>GPGSRYPVRRLPFSTVSKQDLAAFERIVPGGVVTDPEALQAPNVDWLRTLRGCSKVLLRPRTSEEVSHILRHCHERNLAVNPQGGNTGMVGGSVPVFDEIILSTARMNRVLSFHSVSGILVCQAGCVLEELSRYVEERDFIMPLDLGAKGSCHIGGNVATNAGGLRFLRYGSLHGTVLGLEVVLADGTVLDCLTSLRKDNTGYDLKQLFIGSEGTLGIITTVSILCPPKPRAVNVAFLGCPGFAEVLQTFSTCKGMLGEILSAFEFMDAVCMQLVGRHLHLASPVQESPFYVLIETSGSNAGHDAEKLGHFLEHALGSGLVTDGTMATDQRKVKMLWALRERITEALSRDGYVYKYDLSLPVERLYDIVTDLRARLGPHAKHVVGYGHLGDGNLHLNVTAEAFSPSLLAALEPHVYEWTAGQQGSVSAEHGVGFRKRDVLGYSKPPGALQLMQQLKALLDPKGILNPYKTLPSQAHHHHHH[2x]

Human D-2-HGDH is a member of the 2-hydroxy acid dehydrogenase subfamily of the VAO/PCMH flavoprotein family. Regardless of their promiscuous metabolic origins, D-2-HG and L-2-HG can be converted back to 2-OG by two mitochondrial enzymes in humans, namely D-2-HG and L-2-HG dehydrogenases (D-2-HGDH and L-2-HGDH). Like other members of the VAO/PCMH flavoprotein family, D-2-HGDH is comprised of two major domains named the FAD-binding domain and the substrate-binding domain supplemented with a small C-terminal domain. The active site resides at the interface of the FAD-binding domain and the substrate-binding domain, and consists of the FAD-binding site and the substrate-binding site.

Crystallization of D-2-HGDH in the absence of any ligands yielded crystals of D-2-HGDH in apo form. Structure of the apo D-2-HGDH was solved at 2.20 Å resolution, and structures of D-2-HGDH in complexes with D-2-HG, D-MAL, D-LAC, L-2-HG, and 2-OG were solved at 2.65 Å, 2.80 Å, 2.62 Å, 3.00 Å, and 2.80 Å resolution, respectively. The asymmetric unit contains two D-2-HGDH molecules with essentially identical conformation. In all the structures, there is a FAD non-covalently bound to the active site, which is apparently co-purified with the enzyme, indicating that D-2-HGDH binds FAD tightly. In the apo D-2-HGDH structure, there is no metal ion or ligand bound at the active site. In the apo structure, the substrate-binding site is occupied by several water molecules; in the D-2-HG-bound structure, there are a Zn2+ and a D-2-HG bound at the substrate-binding site. The structural comparison shows that the binding of Zn2+ and D-2-HG does not induce notable conformational changes at the substrate-binding site as well except for Glu475 which adopts a different side-chain conformation to interact with the Zn2+. In all the D-2-HGDH structures, the FAD assumes an elongated conformation with the isoalloxazine ring in a distal position from the AMP moiety.> AESTLGAAAAQSGRYFGTAIASGKLGD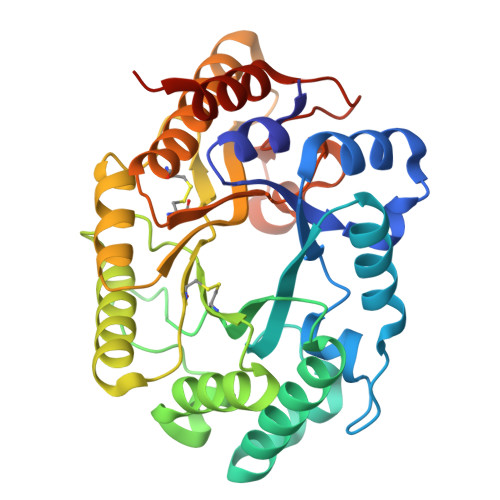SAYTTIASREFNMVTAENEMKIDATEPQRGQFNFSAGDRVYNWAVQNGKQVRGHTLAWHSQQPGWMQSLSGSTLRQAMIDHINGVMGHYKGKIAQWDVVNEAFSDDGSGGRRDSNLQRTGNDWIEVAFRTARAADPAAKLCYNDYNIENWTWAKTQGVYNMVRDFKQRGVPIDCVGFQSHLIVGQVPGDFRQNLQRFADLGVDVRITELDIRMRTPSDATKLATQAADYKKVVQACMQVTRCQGVTVWGITDKYSWVPDVFPGEGAALVWDASYAKKPAYAAVMEAFGSRSHHHHHH N-METHYLACETAMIDE | C3 H7 N O | 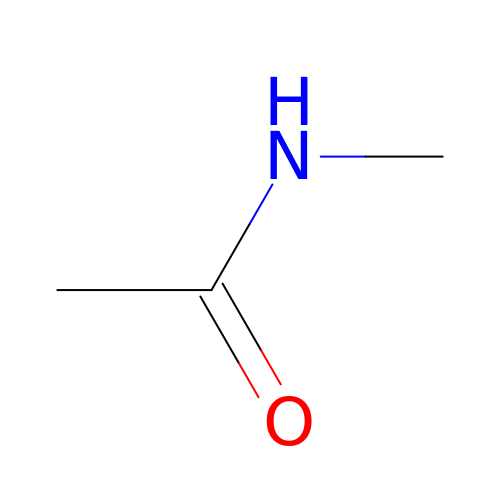OHLUUHNLEMFGTQ-UHFFFAOYSA-N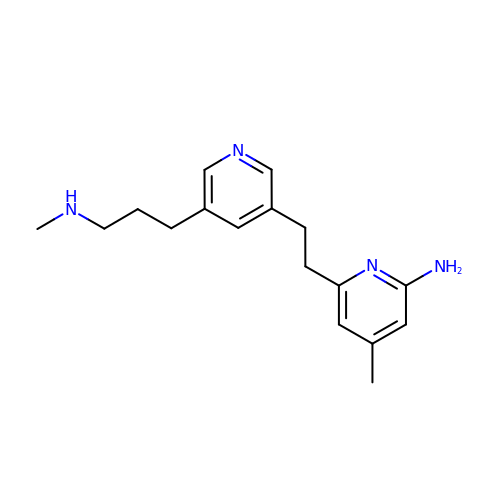4-METHYL-6-(2-(5-(3-(METHYLAMINO)PROPYL)PYRIDIN-3-YL)ETHYL)PYRIDIN-2-AMINE | C17 H24 N4 | YUXWMCKGSHXUGW-UHFFFAOYSA-N> PISPIETVPVKLKPGMDGPKVKQWPLTEEKIKALVEICTEMEKEGKISKIGPENPYNTPVFAIKKKDSTKWRKLVDFRELNKRTQDFWEVQLGIPHPAGLKKNKSVTVLDVGDAYFSVPLDEDFRKYTAFTIPSINNETPGIRYQYNVLPQGWKGSPAIFQSSMTKILEPFKKQNPDIVICQYMDDLYVGSDLEIGQHRTKIEELRQHLLRWGLTTPDKKHQKEPPFLWMGYELHPDKWTVQPIVLPEKDSWTVNDIQKLVGKLNWASQIYPGIKVRQLSKLLRGTKALT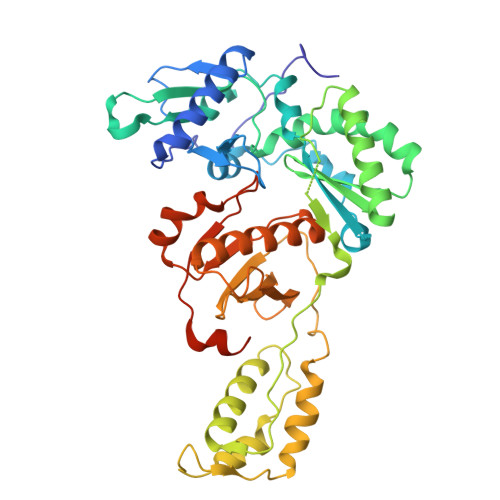EVIPLTEEAELELAENREILKEPVHGVYYDPSKDLIAEIQKQGQGQWTYQIYQEPFKNLKTGKYARMRGAHTNDVKQLTEAVQKITTESIVIWGKTPKFKLPIQKETWETWWTEYWQATWIPEWEFVNTPPLVKLWYQLEKEPIVGAETFYVDGAAN> MATVLLAAAGGAIGTSLGGALFGISAAVIGQAVGGLIGQTIDARLSGGGTIKQTGPRLDSLEVMVSQEGTPLADISGRVAVAGTVIWATKLEEIARTTSTRVGSGKSSQKVKSTNFDYAASFAVSLGEGPLNGIGRIFLDGQVRDLSEMISENRVRFYPGTEDQEPDPLIEAIEGAAPAFRGTAYLVFERLFLSDFGNRVPQVRVEVFGQSGEMEKGVTGVCVIPGSTEFGYMPAPVRQQSLDGADVVWEGPENCNRYSRISDWSLSMDHLKNTLPAVQTVSLVVAWFGTDLRAGLCRFEPRIELRAKRTSIEWIAAGLNRGSATEVSRDENDRPAFGSSPADVSVVRAIMDLKARGFRVVLYPFVMMDVTADQALPSPAGTGAQGAYPWRGRIMPDVTGGRVSDQIAALMGTAQPDDFTAAVTRNKSGEISQVNLTCPGAPGDAGLRRFILHLAKLADIAGGVDAFLVGTEFRGLSQAWEPQTYADAYEFLNSSEGWFAQNAARTHEPGSLLVSATARDPRLISPPLSIDGAAARWIEIEFDRTSAPVWEGNVYYMTEDHGFAGAFRKVISDAEAPADGTRARMLLDMHDLTLGGDDWRTSTITRLRFDFSSESDAVFRIHAIRLGGGRRYPFVDALRDLAQDVDTILPTAKISYAADWSEYHSHQDAGDLTFHLDPLWADPAIDFVGIDNYLPLSDWRQGADHLDYDATSGRTTPYDLDYLKSNIEGGEYWDWFYASQEDRDTQTRTPISDGSYGEPWVFRQKAIRDWHANAHHNRTAGVRATTSTGWVPGSKPVWFTEYGCPAVDLGANRPNVFAAASSSESALPWYSSGLRDDFMQRQYLRAMAEWWTANGAPAVDLANCQAWAWDARPFPEFPLRPATWSDGPDWRLGHWLNGRAGAAPAAEAITRRAITRHGLISADIDTSRAYGQADGYAAPAPLGLGDYAQPFEVALGLQTTETGGALVIEAKPAAPLAADVIEADLVDTPAIYTLTRGALEDTPAAAIVRFRDGLSDYEITAARARI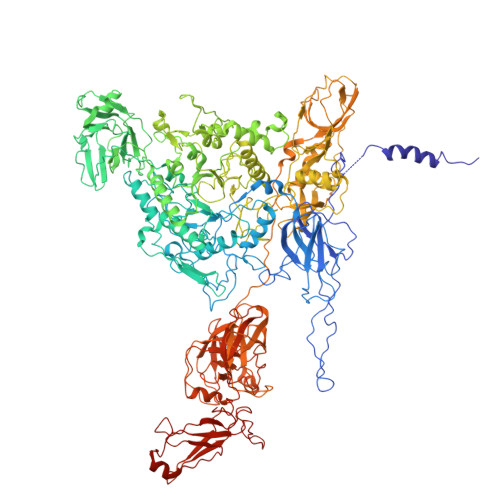GAGKEGGSATADLALVLDGDRGNAAAEMVLRAALTSRESLSVTLPRSATTLRPGSLVEVTLGTEARRLFLVDRVVDGQAREVTLRGFDRAAYAPSGGVFKAARAGRLQGSTSSLTRFLDLPLLPGVDAPEWEGFIAAHAEPWPGAMLHSRGSTPEGSFTLAAEADARATIGRTTAALPPAPAHVWTPGPLVVTLFSGALVGRPDLDVLDGANALAIQHPDGWEVVQFREATLTADRTWRLEGLLRGQRGTDGIVGPAPLPAGAAVVAIDTALVAAGLSADDPGRALWWRSGPDAASLAAAPLRPHTFTAAGLRAFPPAHLRAVVTGGGDTSLSWVPRSRLVGTTWPDNGAPIPSGEGLERYQVTIGPTAAPVRVILADTPAATYTAAERAADGIAAPFRVAVSQISETTGPGPWIETIVTE> MTAILALLLAMSILLPSGAVEDVQDLVFAEWDKGSSHEHACSALRNSSVIEKGLTVKEVGTSKFAAVLSEPILARLKFHGLVEAVPVVEVGTVMKRLNVSIPPAQDISDNNLTLIKMSPKLKGQTLQQIDAELRYLGEYMNTVLQKCSHRVYISKGTFPPKIYVFLNMPLDQ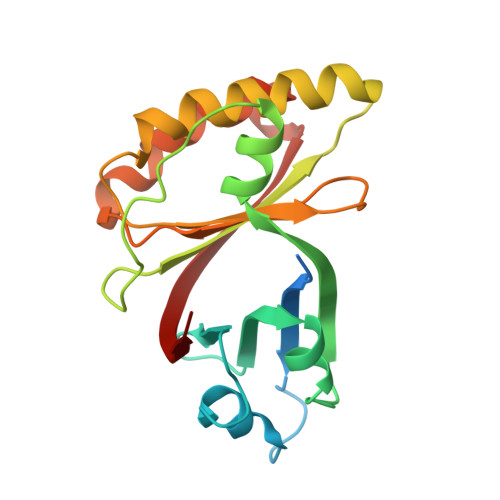IRQFYPSLDIFGGPSSTKNEISYVQILILRN>[2x]PPRGKTVWFTGLSGSGKSSVAMLVERKLLEKGISAYVLDGDNLRHGLNADLGFSMADRAENLRRLSHVATLLADCGHLVLVPAISPLAEHRALARKVHAD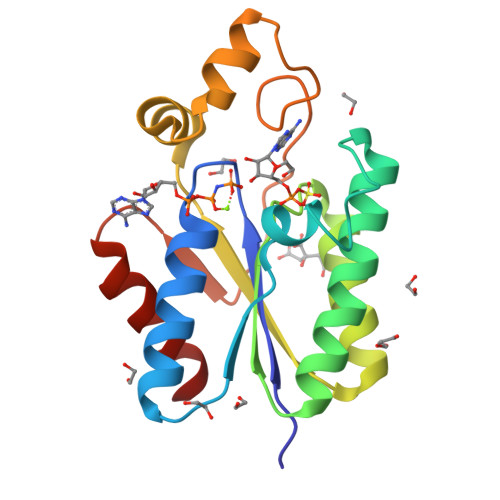AGIDFFEVFCDTPLQDCERRDPKGLYAKARAGEITHFTGIDSPYQRPKNPDLRLTPDRSIDEQAQEVIDLLES> GAMGSGIQRPTSTSSLVAAAMAEEEEVEEGRSSSSAILDLPEPLLLHILSFLTDVRSRHRAALACG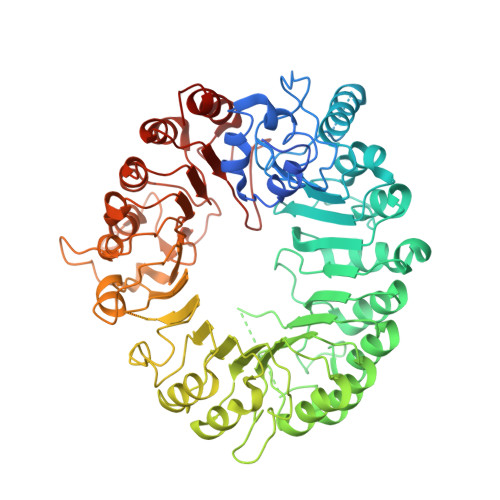RMRAAERATRSELSLRGDPRSPGFLFLSHAFRFPALEHLDLSLVSPWGHPLLSSVPPCGGGGGGAPSASSSSGMNVYHPEAISEQNAFIAARLAGCFPAVTSLAVYCRDPTTLANLTPHWQASLRRVKLVRWHQRPPTLPDGADLEPLLETCAALRELDLSEFYCWTEDVVRALTTHPSATAALTHLDLGLAAATDGFKSSELGPIAASCPNLRKLVAPCLFNPRFSDCVGDDALLSLATSCPRLTVLRLSEPFEAAANIQREEAAITVAGLVAFFAALPALEDFTMDLQHNVLEAAPAMEALARRCPRIKFLTLGSFQGLCKASWLHLDGVAVCGGLESLYMKNCQDLTDASLAAIGRGCRRLAKFGIHGCDLVTSAGIRRLAFTLRPTLKEVTVLHCRLLHTAECLTALSPIRDRIESLEINCVWNTTEQPCSVANGTTTECDPEDDELGEVYESAAKKCRYMEFDDLGSWEMLRSLSLWFSAGQLLSPLISAGLDSCPVLEEISIKVEGDCRTCPRPAPRTIFGLSDLAGFPVLAKMKLDLSEAVGYALTAPTGQMDLSLWERFYLHGIESLQTLYELDYWPPQDKDVHHRSLTLPAVGLIQRCVGLRKLFIHGTTHEHFMTFFLSIPNLRDMQLREDYYPAPENDLMFTEMRAESWLRFEVQLNSRQIDD>FNLPLGNYKKPKLLYCSNGGYFLRILPDGTVDGTKDRSDQHIQLQLAAESIGEVYIKSTETGQFLAMDTDGLLYGSQTPNEECLFLERLEENGYNTYISKKHAEKHWFVGLKKNGRSKLGPRTHFGQKAIL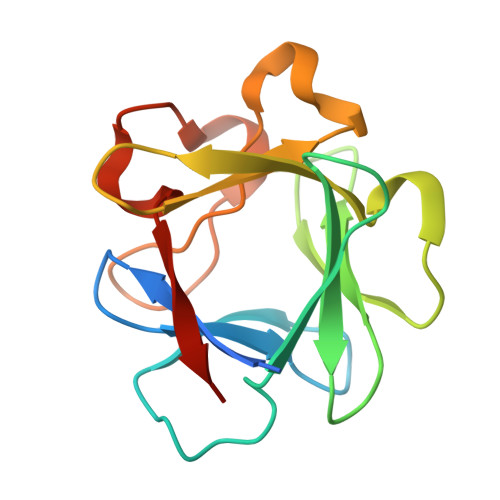FLPLPVSSD[2x]>MEKRMSTQQRAAGNACPTAAFSFDPARLAQRRRWAGAFAALCGLALSPSALLAEEHSQHQDHAVELAPSVVTGVAQSSPLTIVTNPKEPRQPVPASDGADYLKTIPGFAVIRNGGSNGDPVLRGMFGSRLNILTNGGMMLGACPNRMDAPTSYISPETYDKLTVIKGPQTVLWGPGASAGTILFEREPERFGELGSRVNASLLAGSNGRFDKVLDAAAGNRLGYLRFTGNHAQSDDYEDGAGNTVPSRWKKWNGDVAVGWTP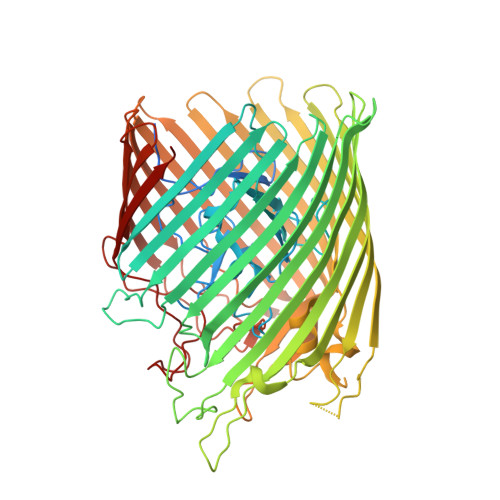DEDTLIELTAGKGDGEARYAGRGMDGSQFKRESLGLRFVKSNVSDVLEKVEAQVYYNYADAIMDNFRLRTPDPSSMMPMPMASQVDRRTLGGRLAATWRWDDFKLVTGVDAMRNEHRARGSKYDMMTDYYTDADQFPWSKDAVFHNYGAFGELTWFAAERDRLIGGLRLDRASVKDYRQTLKSGHMGHAMANPTANDTRADTLPSGFVRYEHDLADSPTTLYAGLGHAERFPDYWELFSPKRGPNGSVNAFDKIKPEKTTQLDFGLQYNGDKLQAWASGYVGVVQDFILFSYREGMMGSSTQATNVDARIMGGELGASYQLTGNWKTDASLAYAWGKNSSDDRALPQIPPLEARFGLTYEEGDWSAGSLWRVVAPQNRIARDQGNVVGKDFDKSAGFGVFSLNGAYRVTRNVKLSAGVDNLFDKDYTEHLNKAGDAGFGFSANETVPEPGRTFWTKVDFSF[4x]> GMPIIIDKDLPARKVLQEENIFVMTKERAETQDIRALKIAILNLMPTKQETEAQLLRLIGNTPLQLDVHLLHMESHLSRNV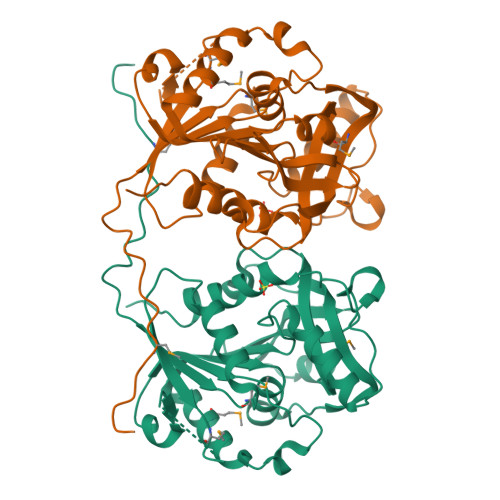AQEHLTSFYKTFRDIENEKFDGLIITGAPVETLSFEEVDYWEELKRIMEYSKTNVTSTLHICWGAQAGLYHHYGVQKYPLKEKMFGVFEHEVREQHVKLLQGFDELFFAPHSRHTEVRESDIREVKELTLLANSEEAGVHLVIGQEGRQVFALGHSEYSCDTLKQEYERDRDKGLNIDVPKNYFKHDNPNEKPLVRWRSHGNLLFSNWLNYYVYQETPYVL> GSSSWNDIKNSGYISRYLTDFEPIQCLGRGGFGVVFEAKNKVDDCNYAIKRIRLPNRELAREKVMREVKALAKLEHPGIVRYFNAWLEAPPEKWQEKLQPSSPKVYLYIQMQLCRKENLKDWMNGRCTIEERERSVCLHIFLQIAEAVEFLHSKGLMHRNLKPSNIFFTMDDVVKVGDFGLVTAMDQDEEEQTVLTPMPAYARHTGQVGTKLYMSPEQIHGNSYSHKVDIFSLGLILFELLYPFSTQMERVRTLTDVRNLKFPPLFTQKYPCEYVMVQDMLSPSPMERPEAINIIENAVFEDLDFPGKTVLRQRSRS

The protein kinase R (PKR)-like endoplasmic reticulum kinase (PERK) is one of three endoplasmic reticulum (ER) transmembrane sensors of the unfolded protein response (UPR) responsible for regulating protein synthesis and alleviating ER stress. Upon activating the UPR, PERK phosphorylates eIF2a at Ser51, leading to widespread inhibition of protein translation with a few selected regulatory proteins translated to restore homeostasis and alleviate ER stress. Herein, we report the synthesis and discovery of a series of novel mandelamide-derived pyrrolopyrimidines (I) that are highly potent, selective, and orally bioavailable PERK inhibitors. These medicinal chemistry efforts were iteratively supported by an X-ray crystallography structure-based approach to develop and refine SAR information.

Hydroxyl substitution on this group was found to increase potency by 2-3-fold (13 vs. 14) with preference for the (R)-over the (S)-enantiomer (11 vs. 12). Compound 11 formed three hydrogen bonds directly with the carbonyl of Q889, the amide of C891, and the carbonyl of F956 from PERK, respectively. In addition, compound 11 forms two hydrogen bonds with a water molecule, and this molecule hydrogen bonds to the amide of V652. In the ATP binding hinge region, substitution at the C2-position (R1) of the pyrrolopyrimidine ring appeared feasible, filling a small pocket near C891. Compounds 11 and 24 were screened in the DiscoverX scanMAXSM panel of 468 kinases. The resulting TREEspotTM interaction maps revealed that the methyl substituent in 24 led to superior selectivity versus 11. The S(35), S(10), and S(1) selectivity scores at a concentration of 1 µM were 0.005, 0, and 0 for 24 versus 0.072, 0.035, and 0 for 11. Given the superior selectivity of 24 but slight loss in potency versus 11, further optimization of the series was carried out with the 2-methyl substitution on the pyrrolopyrimidine ring to further improve potency and drug-like properties.(3Z)-3-({3,5-dimethyl-4-[(4-methylpiperidin-4-yl)carbamoyl]-1H-pyrrol-2-yl}methylidene)-2-oxo-N-[(1R)-1-phenylethyl]-3,7-dihydro-2H-indole-5-carboxamide 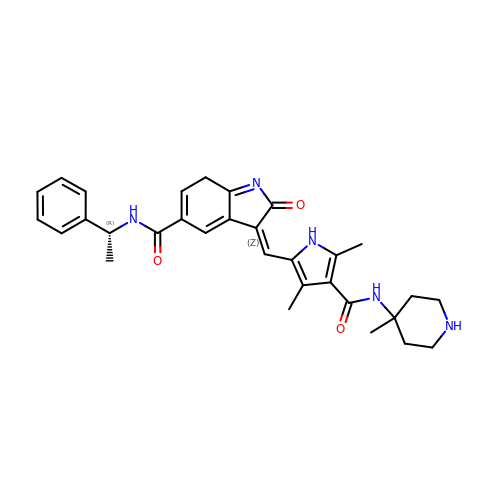| C31 H35 N5 O3 | ZDUMEWZQRJWZEW-RJDQKLELSA-N N-[3-[(5R)-3-azanyl-5-methyl-9,9-bis(oxidanylidene)-2,9$l^{6}-dithia-4-azaspiro[5.5]undec-3-en-5-yl]-4-fluoranyl-phenyl]-5-(fluoranylmethoxy)pyrazine-2-carboxamide 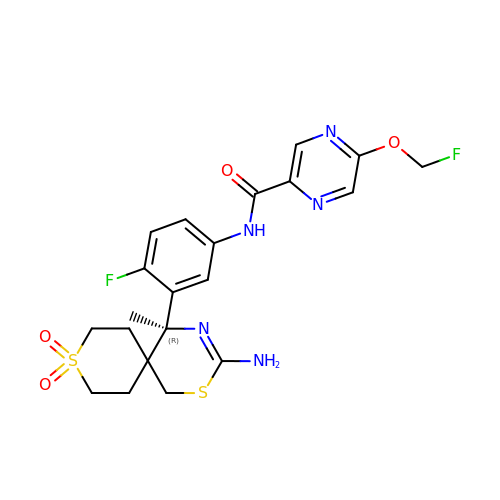| C21 H23 F2 N5 O4 S2 | DZTJZUAOGBUBNK-HXUWFJFHSA-N>GSAPPGDPVEGKHLFHTICITCHTDIKGANKVGPSLYGVVGRHSGIEPGYNYSEANIKSGIVWTPDVLFKYIEHPQKIVPGTKMGYPGQPDPQKRADII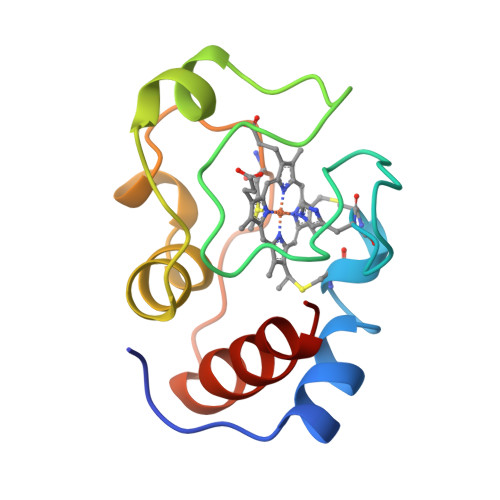AYLETLK[2x]MPO is a heme Fe3+-containing peroxidase with a protoporphyrin IX as the basic structure of its prosthetic group. The porphyrin ring of MPO is covalently attached to the enzyme via two ester bonds (Asp260 and Glu408) and one electron-withdrawing sulfonium linkage (Met409), and features a histidine as a proximal ligand (His502). When neutrophilic polymorphonuclear leukocytes (neutrophils) entrap microbial or other invasive particulates, they release MPO during degranulation.

Here, we present a new crystal form containing four homodimers of human MPO at 2.6 Å resolution. We could capture the binding of the serotonin-transporter inhibitor paroxetine, which is known to be one of the few irreversible MPO inhibitors, in the crystal structure of the native enzyme. Clear electron density is present for paroxetine bound in four of the eight monomers of MPO. The entries to the four other catalytic sites are obstructed by an arginine residue (Arg653) that inserts between the side chain of Asp384, with which it makes a salt bridge, and the carbonyl group of Val576. Every MPO homodimer has only one paroxetine bound and this is with a partial occupancy of paroxetine ranging from 1.0 (full occupancy) in chain A to 0.73 (partial occupancy) in chain H. The reason for the non­saturation of MPO by paroxetine is probably because of its lower concentration (25 µM) compared with MPO (138 µM) in the crystallization condition. Thiocyanate, in its negatively charged form SCN−, can bind MPO and oxidize to HOSCN, which can induce reversible modifications to mammalian cells that are repairable and thus less damaging. In our crystal structure, thiocyanate is found in the same position hovering above the heme porphyrin ring. The final model contains eight polypeptide chains of mature MPO and 30 glycan chains on an asparagine side-chain ND2 atom, or in brief N-glycosylation.

>TCPEQDKYRTITGMCNNRRSPTLGASNRAFVRWLPAEYEDGFSLPYGWTPGVKRNGFPVALARAVSNEIVRFPTDQLTPDQERSLMFMQWGQLLDHDLDFTPEPAARASFVTGVNCETSCVQQPPCFPLKIPPNDPRIKNQADCIPFFRSCPACPGSNITIRNQINALTSFVDASMVYGSEEPLARNLRNMSNQLGLLAVNQRFQDNGRALLPFDNLHDDPCLLTNRSARIPCFLAGDTRSSEMPELTSMHTLLLREHNRLATELKSLNPRWDGERLYQEARKIVGAMVQIITYRDYLPLVLGPTAMRKYLPTYRSYNDSVDPRIANVFTNAFRYGHTLIQPFMFRLDNRYQPMEPNPRVPLSRVFFASWRVVLEGGIDPILRGLMATPAKLNRQNQIAVDEIRERLFEQVMRIGLDLPALNMQRSRDHGLPGYNAWRRFCGLPQPETVGQLGTVLRNLKLARKLMEQYGTPNNIDIWMGGVSEPLKRKGRVGPLLACIIGTQFRKLRDGDRFWWENEGVFSMQQRQALAQISLPRIICDNTGITTVSKNNIFMSNSYPRDFVNCSTLPALNLASWREA[8x]> EWEALE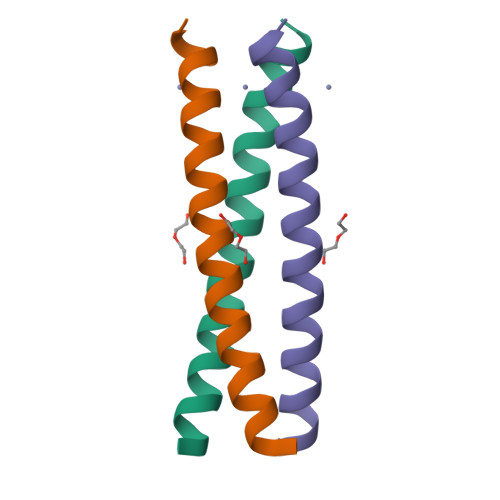KKLAALESKCQALEKKLQALEKKLEALEHG>[5x]MITVIAIAKDGSIVEPKLDEISFEDYRLIWIDCYDPKDEELYKLSKKIGISVSDLQIGLDEQEIPRVEEDEDFYLIIYKAPLFEEDITTTSLGIYIKNNLLLTIHSDKIKAIGRLHKLISTKKPRIVFERGIGFLLYHILNEITRSYSRILMNLEDELEELEDKLLAGYDREVMEKILGLRKTLVYFHKSLIANRDVLVLLKRKYLPITTKEDRENFEDLYYDTLQLIDMSATYREVLTSMMDITLSLENIKMNQIMKILTMVTTIFAVPMWITGIYGMNFSYLPLANNPQGFWLVMALMVVIIMIFVYIFRRSGWI

The CorA proteins are ion channels having a major role in the flux of magnesium ions across the cytoplasmic membrane in prokaryotes. CorA channels are homo-pentameric with a large cytoplasmic domain and a smaller trans-membrane (TM) domain. CorA channels have a gate formed by an annulus of hydrophobic residues coincident with the inner membrane surface and [15], [16], in the structures of CorA channels determined to date the dimensions of this gate region would block the passage of magnesium ions through the channel. Gating of the CorA channel to modulate ion conduction is thought to occur through conformational changes in the CorA protein which in turn are moderated by the binding of divalent ions.

In order to further analyse the open state of the CorA channel, we have integrated lower-resolution studies of MjCorA using Small Angle X-ray Scattering and Single Particle Cryo-Electron Microscopy in the absence of magnesium and combined these with low resolution X-ray crystallographic data from crystals grown in low pH conditions disfavouring magnesium binding. The solution conditions for both SAXS and Cryo-EM experiments were similar and in both cases with alkaline buffers lacking Mg2+ ions. The asymmetry of the cytoplasmic domain results from both increased and decreased separations of the channel protomers. The underlying drivers for change in channel conformation are likely to be due to two factors: (1) a replacement of chelating ions with monodentate ligating ions allowing increased protomer separation, and (2) the formation of salt bridges between protomers, acting to decrease protomer separation. The most informative model was determined to be the combination of 3 asymmetric MjCorA pentamers of the form ttrrr, tttrr and ttttr. Taut conformations of an isolated protomer are not seen, taut conformations are present only with two or more adjacent protomers. In the simple rigid body modelling applied here the r protomer conformation leads to an increased displacement of the YGMNF motif from the pore axis, whereas this displacement is reduced for t conformations. The separation of the TM domains at low Mg2+ tension seen here indicates that Mg2+ stabilizes this TM oligomer, and that in vivo in the membrane the close association of TM domains seen in the crystal structures would be re-established by extracellular Mg2+. The study reported here indicates that this asymmetry would be consistent with an increased admittance by the TM segment of the MjCorA channel and improved access to ion binding sites between channel domains in the cytoplasm.Fatty-acid photodecarboxylase (FAP), together with protochlorophyllide oxidoreductase and DNA photolyases, is a member of the rare class of photoenzymes that require light to initiate each catalytic event. Absorption of a blue-light photon by the flavin adenine dinucleotide (FAD) cofactor within FAP triggers the decarboxylation of the fatty-acid substrate, which leads to the formation of a hydrocarbon molecule and CO2. The recently published high-resolution (1.8 Å) structure of FAP, determined from cryo-crystallo­graphic synchrotron data combined with UV–Vis absorbance spectra, revealed a bent oxidized FAD in the dark state. Forward electron transfer from the fatty-acid substrate to the photoexcited FAD occurs in 300 ps and is accompanied by concomitant decarboxylation of the latter, as shown by time-resolved visible and infrared (IR) absorption spectroscopies, respectively.

Here, we extend the study of Sorigué et al. by carrying out the refinement of intermediate-state structures against extrapolated structure factors at 20 ps, 900 ps, 300 ns and 2 µs. In order to model the structural changes that had occurred at the different time points, structure-factor extrapolation was carried out using Xtrapol8, which estimates the structure-factor amplitudes F ext that would have been measured for each pump–probe data set if the photo-triggered intermediate were present in the crystals at 100% occupancy (equation 1). The occupancy of intermediate states was determined to be between 25% and 35% for the four time delays.

>SSPVAQKYDYILVGGGTAACVLANRLSADGSKRVLVLEAGPDNTSRDVKIPAAITRLFRSPLDWNLFSELQEQLAERQIYMARGRLLGGSSATNATLYHRGAAGDYDAWGVEGWSSEDVLSWFVQAETNADFGPGAYHGSGGPMRVENPRYTNKQLHTAFFKAAEEVGLTPNSDFNDWSHDHAGYGTFQVMQDKGTRADMYRQYLKPVLGRRNLQVLTGAAVTKVNIDQAAGKAQALGVEFSTDGPTGERLSAELAPGGEVIMCAGAVHTPFLLKHSGVGPSAELKEFGIPVVSNLAGVGQNLQDQPACLTAAPVKEKYDGIAISDHIYNEKGQIRKRAIASYLLGGRGGLTSTGCDRGAFVRTAGQALPDLQVRFVPGMALDPDGVSTYVRFAKFQSQGLKWPSGITMQLIACRPQSTGSVGLKSADPFAPPKLSPGYLTDKDGADLATLRKGIHWARDVARSSALSEYLDGELFPGSGVVSDDQIDEYIRRSIHSSNAITGTCKMGNAGDSSSVVDNQLRVHGVEGLRVVDASVVPKIPGGQTGAPVVMIAERAAALLTGKATIGASAAAPATVAA[2x]>[12x]MPHSYPALSAEQKKELSDIALRIVAPGKGILAADESVGSMAKRLSQIGVENTEENRRLYRQVLFSADDRVKKCIGGVIFFHETLYQKDDNGVPFVRTIQDKGIVVGIKVDKGVVP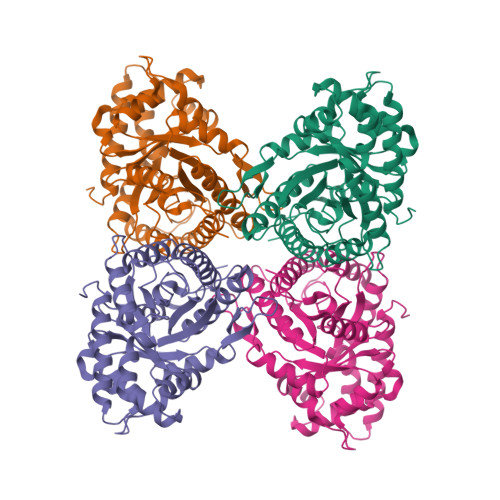LAGTDGETTTQGLDGLSERCAQYKKDGADFAKWRCVLKISERTPSALAILENANVLARYASICQQNGIVPIVEPEILPDGDHDLKRCQYVTEKVLAAVYKALSDHHVYLEGTLLKPNMVTPGHACPIKYTPEEIAMATVTALRRTVPPAVPGVTFLSGGQSEEEASFNLNAINRCPLPRPWALTFSYGRALQASALNAWRGQRDNAGAATEEFIKRAEVNGLAAQGKYEGSGEDGGAAAQSLYIANHAYL>[2x]MAEAGITGTWYNQLGSTFIVTAGADGALTGTYESAVGN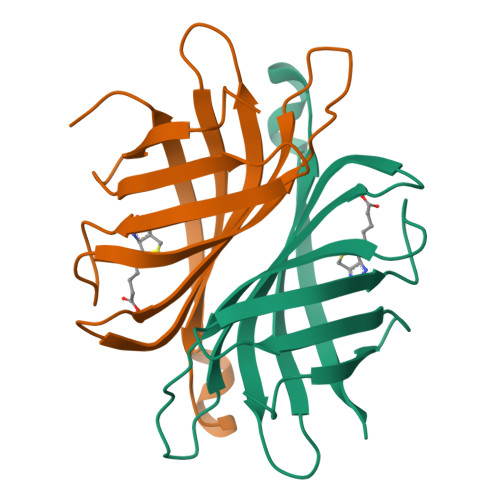AESRYVLTGRYDSAPATDGSGTALGWTVAWKNNYRNAHSATTWSGQYVGGAEARINTQWLLTXGTTEANAWKSTLVGHDTFTKVKPSAASLEHHHHHH> TMLSFVTTDANIDHGHLQGALSAITNETFNRITVDGDTSTNDMVVVMASGLAENETLTPEHPDWANFYKALQL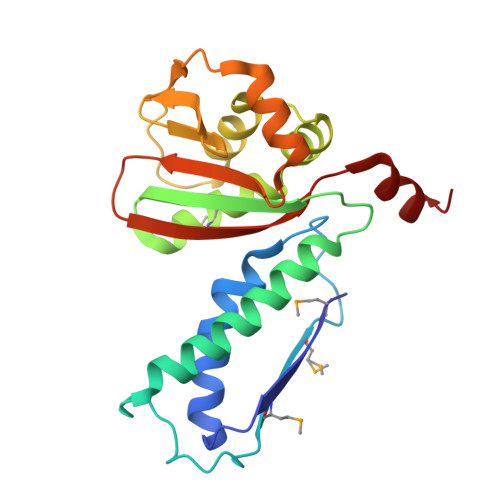ACEDLAKQIARDGEGATKLIEVEVTGAANDQEAGMVAKQIVGSDLVKTAIYGADANWGRIICAIGYSGCEVNQETIDIAIGPIVTLKQSEPTGFSEEEATAYLKEADPVKISVNLHIGNGTGKAWGCDLTYDYVRINAGYRT>PMFIVNTNVPRASVPDGFLSELTQQLAQATGKPPQYIAVHVVPDQLMAFGGSSEPCALCSLHSIGKIGGAQNRSYSKLLCGLLAER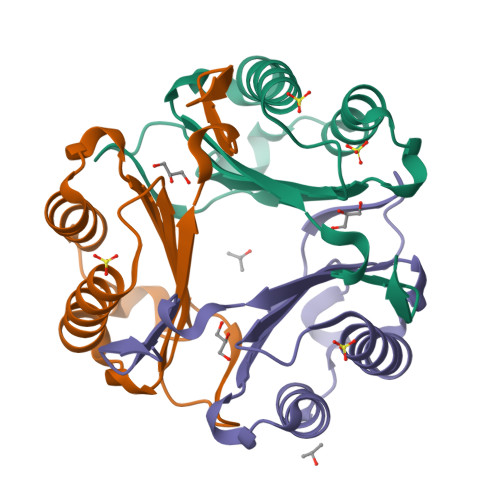LRISPDRVYINYYDMNAANVGWNASTFA[3x]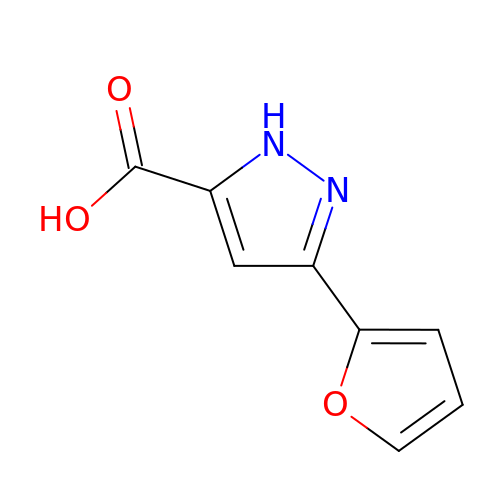3-(furan-2-yl)-1H-pyrazole-5-carboxylic acid | C8 H6 N2 O3 | GKPSFQIKCROJOB-UHFFFAOYSA-N CARBOBENZYLOXY-(L)-LEUCINYL-(L)LEUCINYL METHOXYMETHYLKETONE | C22 H36 N2 O5 | 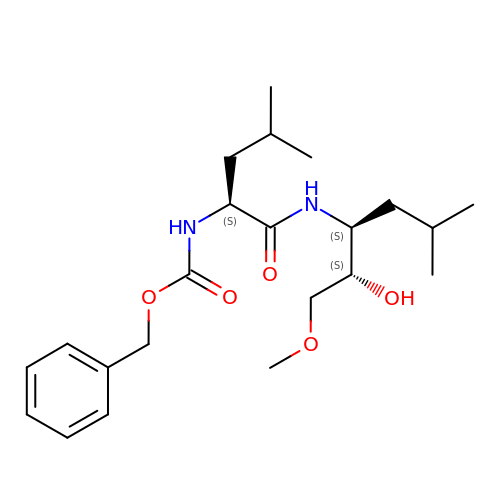LHCNZPLAATYYPI-SLFFLAALSA-N> AMRYGQSPNMPSR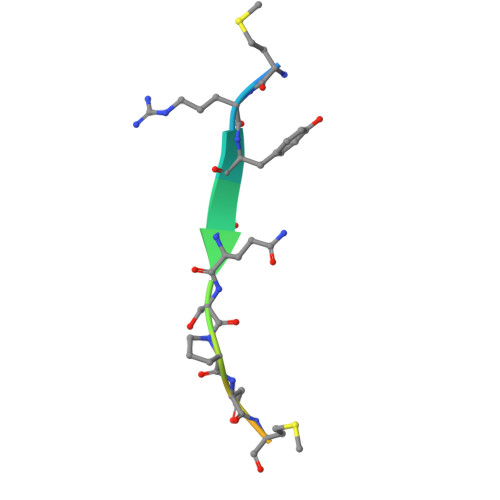RGN>MTVTLAGNPIEVGGHFPQVGEIVENFILVGNDLADVALNDFASKRKVLNIFPSIDTGVCATSVRKFNQQAAKLSNTIVL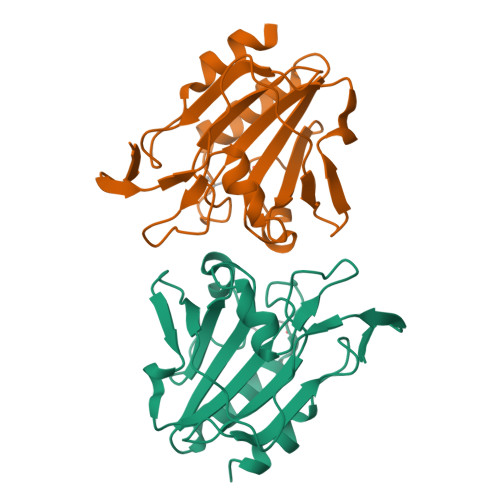CISADLPFAQARFCGAEGIENAKTVSTFRNHALHSQLGVDIQTGPLAGLTSRAVIVLDEQNNVLHSQLVEEIKEEPNYEAALAVLA[2x]> STDNAETGVIEAGNTDTDFSGELAAPGSNHTNVKFLFDRSRLLNVIKVLEKDAVFPRPFPTQEGAQQDDGYFCLLTPRPTVASRPATRFGLYANPSGSGVLANTSLDFNFYSLACFTYFRSDLEVTVVSLEPDLEFAVGWFPSGSEYQASSFVYDQLHVPFHFTGRTPRAFASKGGKVSFVLPWNSVSSVLPVRWGGASKLSSATRGLPAHADWGTIYAFVPRPNEKKSTAVKHVAVYIRYKNARAWCPSMLPFRSYK;> GPIPTAPRENSLMFLSTLPDDTVPAYGNVRTPPVNYLPGEITDLLQLARIPTLMAFERVPEPVPASDTYVPYVAVPTQFDDRPLISFPITLSDPVYQNTLVGAISSNFANYRGCIQITLTFCGPMMARGKFLLSYSPPNGTQPQTLSEAMQCTYSIWDIGLNSSWTFVVPYISPSDYRETRAITNSVYSADGWFSLHKLTKITLPPDCPQSPCILFFASAGEDYTLRLPVDCNPSYVF;> DRVTTQTAGNTAINTQSSLGVLCAYVEDPTKSDPPSSSTDQPTTTFTAIDRWYTGRLNSWTKAVKTFSFQAVPLPGAFLSRQGGLNGGAFTATLHRHFLMKCGWQVQVQCNLTQFHQGALLVAMVPETTLDVKPDGKAKSLQELNEEQWVEMSDDYRTGKNMPFQSLGTYYRPPNWTWGPNFINPYQVTVFPHQILNARTSTSVDINVPYIGETPTQSSETQNSWTLLVMVLVPLDYKEGATTDPEITFSVRPTSPYFNGLRNRYTAG;> RGNNGNMTFNYYANTYQNSVDFSTSSSASGAGPGNSRGGLAGLLTNFSGILNPLGYLK;> CYGGFDLYFILDKSGSVLHHWNEIYYFVEQLAHKFISPQLRMSFIVFSTRGTTLMKLTEDREQIRQGLEELQKVLPGGDTYMHEGFERASEQIYYENRQGYRTASVIIALTDGELHEDLFFYSEREANRSRDLG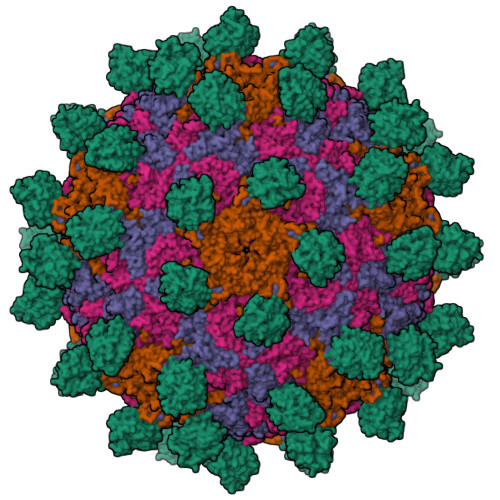AIVYAVGVKDFNETQLARIADSKDHVFPVNDGFQALQGIIHSILKKSC8-[2-azanyl-3-chloranyl-5-(1-methylindazol-5-yl)pyridin-4-yl]-2,8-diazaspiro[4.5]decan-1-one 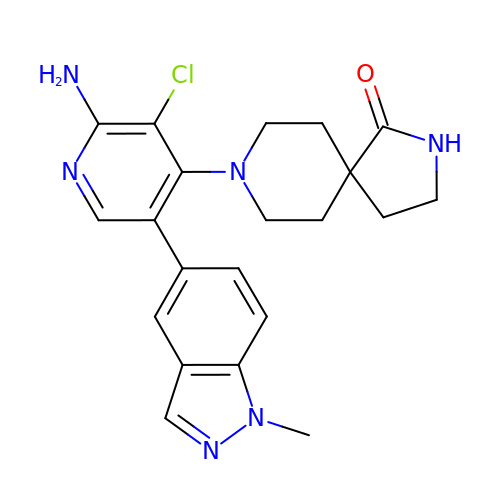| C21 H23 Cl N6 O | VPJXPDLMACOGIZ-UHFFFAOYSA-N>[4x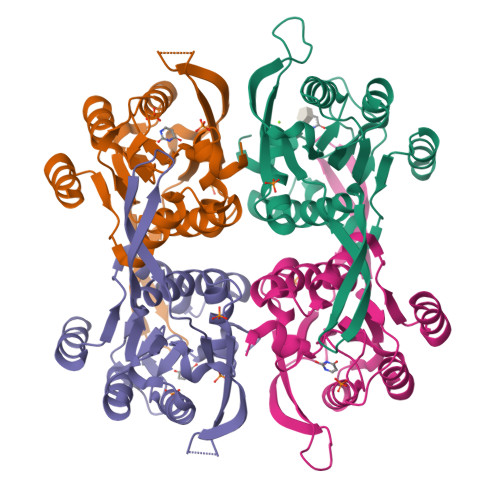]AQVPASGKLLVDPRYSTNDQEESILQDIITRFPNVVLMKQTAQLRAMMTIIRDKETPKEEFVFYADRLIRLLIEEALNELPFQKKEVTTPLDVSYHGVSFYSKICGVSIVRAGESMESGLRAVCRGVRIGKILIQRDETTAEPKLIYEKLPADIRERWVMLLDPMCATAGSVCKAIEVLLRLGVKEERIIFVNILAAPQGIERVFKEYPKVRMVTAAVDICLNSRYYIVPGIGDFGDRYFGTM>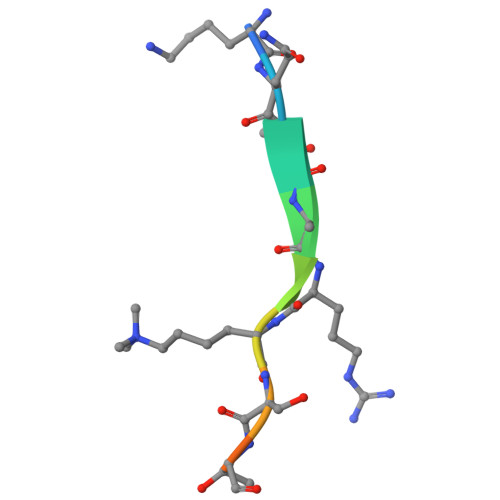 KQTARKSTGGK> MGRVYYGGVERTYLYRGRILNLALEGRYEIVEHKPAVAVIALREGRMLFVRQMRPAVGLAPLEIPAGLIEPGEDPLEAARRELAEQTGLSGDLTYLFSYFVSPGFTDEKTHVFLAENLKEVEAHPDEDEAIEVVWMRPEE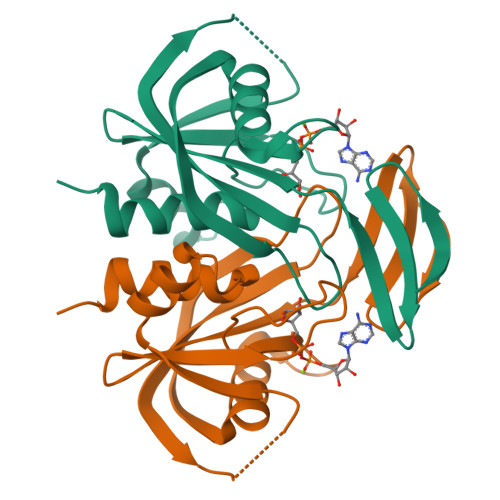ALERHQRGEVEFSATGLVGVLYYHAFLRGR>[2x]SN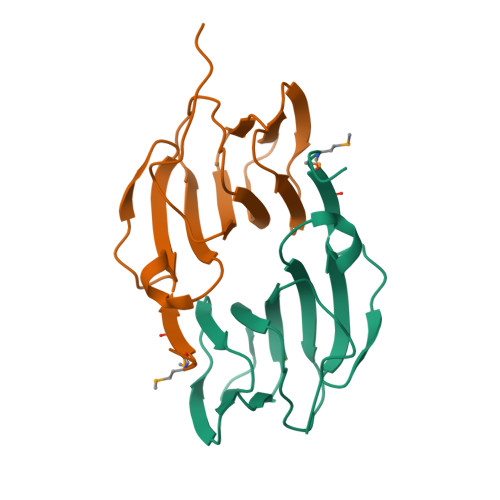AMTESTKDSPSAAMPQMISLSEIEAVACPCGWAQRAFGHDAGTSVSVHYTQITKAARTHYHREHQEIYVVLDHAAHATIELNGQSYPLTKLLAISIPPLVRHRIVGEATIINIVSPPFDPADEWFDSSDMNCDEMNADMNTADTSSALPMEIHHV> MSEMSYLEKLLDGVEVEWLPLGEITKYEQPTKYLVKAKDYHDTYTIPVLTAGKTFILGYTNETHGIYQASKAPVIIFDDFTTANKWVDFDFKAKSSAMKMVTSCDDNKTLLKYVYYWLNTLPSEFAEGDHKRQWISNYSQKKIPIPCPDNPEKSLAIQSEIVRILDKFTALTAELTAELNMRKKQYNYYRDQLLSFKEGEVEWKTLGEIGKWYGGGTPSKNKIEFWENGSIPWISPKDMGRTLVDSSEDYITEEAVLHSSTKLIPANSIAIVVRSSILDKVLPSALIKVPATLNQDMKAVIPHENILVKYIYHMIGSRGSDILRAAKKTGGSVASIDSKKLFSFKIPVPNINEQQRIVEILDKFDTLTNSITEGLPREIELRQKQYEYYRDLLFSFPKPETVSN;>MTHQTHTIAESNNFIVLDKYIKAEPTGDSYQSESDLERELIQDLRNQGYEFISVKSQSAMLANVREQLQNLNGVVFNDSEWRRFTEQYLDNPSDGILDKTRKIHIDYICDFIFDDERLENIYLIDKKNLMRNKVQIIQQFEQAGSHANRYDVTILVNGLPLVQIELKKRGVAIREAFNQIHRYSKESFNSENSLFKYLQLFVISNGTDTRYFANTTKRDKNSFDFTMNWAKSDNTLIKDLKDFTATCFQKHTLLNVLVNYSVFDSSQTLLVMRPYQIAATERILWKIKSSFTAKNWSKPESGGYIWHTTGSGKTLTSFKAARLATELDFIDKVFFVVDRKDLDYQTMKEYQRFSPDSVNGSENTAGLKRNLDKDDNKIIVTTIQKLNNLMKAESDLPVYNQQVVFIFDECHRSQFGEAQKNLKKKFKRYYQFGFTGTPIFPENALGSETTASVFGRELHSYVITDAIRDEKVLKFKVDYNDVRPQFKSLETETDEKKLSAAENQQAFLHPMRIQEITQYILNNFRQKTHRTFPGSKGFNAMLAVSSVDAAKAYYATFKRLQEEAANKSATYKPLRIATIFSFAANEEQNAIGEISDETFDTSAMDSSAKEFLDAAIREYNSHFKTNFSTDSNGFQNYYRDLAQRVKNQDIDLLIVVGMFLTGFDAPTLNTLFVDKNLRYHGLMQAFSRTNRIYDATKTFGNIVTFRDLERSTIDAITLFGDKNTKNVVLEKSYTEYMEGFTDAATGEAKRGFMTVVSELEQRFPDPTS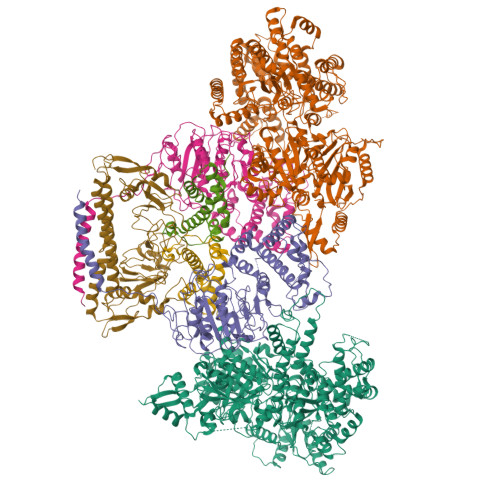IESEKEKKDFVKLFGEYLRAENILQNYDEFATLKALQQIDLSDPVAVEKFKAEHYVDDEKFAELQTIRLPADRKIQDYRSAYNDIRDWQRREKEAEKKEKSTTDWDDVVFEVDLLKSQEINLDYILGLIFEHNRQNKGKGEMIEEVKRLIRSSLGNRAKEGLVVDFIQQTNLDDLPDKASIIDAFFTFAQREQQREAEALIKEENLNEDAAKRYIRTSLKREYATENGTELNETLPKLSPLNPQYKTKKQAVFQKIVSFIEKFKGVGGKI[2x];>[2x]MKMTSIQQRAELHRQIWQIANDVRGSVDGWDFKQYVLGALFYRFISENFSSYIEAGDDSICYAKLDDSVITDDIKDDAIKTKGYFIYPSQLFCNVAAKANTNDRLNADLNSIFVAIESSAYGYPSEADIKGLFADFDTTSNRLGNTVKDKNARLAAVLKGVEGLKLGDFNEHQIDLFGDAYEFLISNYAANAGKSGGEFFTPQHVSKLIAQLAMHGQTHVNKIYDPAAGSGSLLLQAKKQFDNHIIEEGFFGQEINHTTYNLARMNMFLHNINYDKFDIKLGNTLTEPHFRDEKPFDAIVSNPPYSVKWIGSDDPTLINDERFAPAGVLAPKSKADFAFVLHALNYLSAKGRAAIVCFPGIFYRGGAEQKIRQYLVDNNYVETVISLAPNLFFGTTIAVNILVLSKHKTDTNVQFIDASELFKKETNNNILTDAHIEQIMQVFASKEDVAHLAKSVAFETVVANDYNLSVSSYVEAKDNREIIDIAELNAELKTTVSKIDQLRKDIDAIVAEIEGCEVQK;>MAMSNMTYNNVFDHAYEMLKENIRYDDIRDTDDLHDAIHMAADNAVPHYYADIFSVMASEGIDLEFEDSGLMPDTKDVIRILQARIYEQLTIDLWEDAEDLLNEYLEEVEEYEEDEE[2x]6-methyl-4-(piperazin-1-yl)-2-(trifluoromethyl)quinoline | C15 H16 F3 N3 | 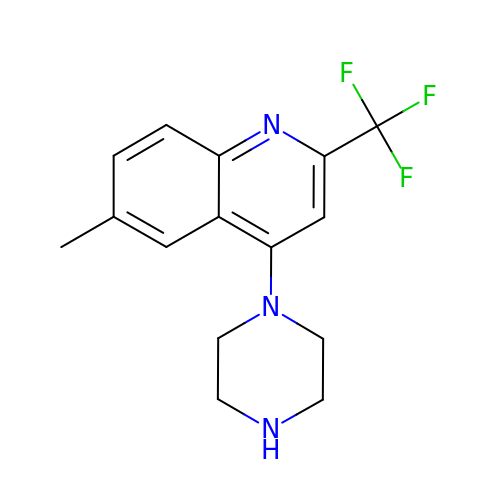ZKHOZLXKYFBVMY-UHFFFAOYSA-N>PVDFTGYWKMLVNENFEEYLRALDVNVALRKIANLLKPDKEIVQDGDHMIIRTLSTFRNYIMDFQVGKEFEEDLTGIDDRKCMTTVSWDGDKLQCVQKGEKEGRGWTQWIEGDELHLEMRVEGVVCKQVFKKVQHHHHHH[3x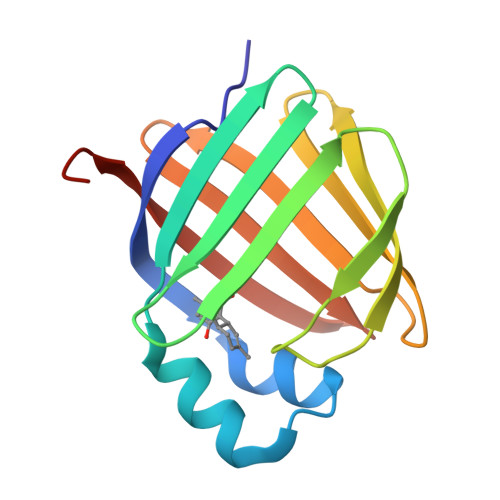]>GAMSAADEVDGLGVARPHYGSVLDNERLTAEEMDERRRQNVAYEYLCHLEEAKRWMEACLGEDLPPTTELEEGLRNGVYLAKLGNFFSPKVVSLKKIYDREQTRYKATGLHFRHTDNVIQWLNAMDEIGLPKIFYPETTDIYDRKNMPRCIYCIHALSLYLFKL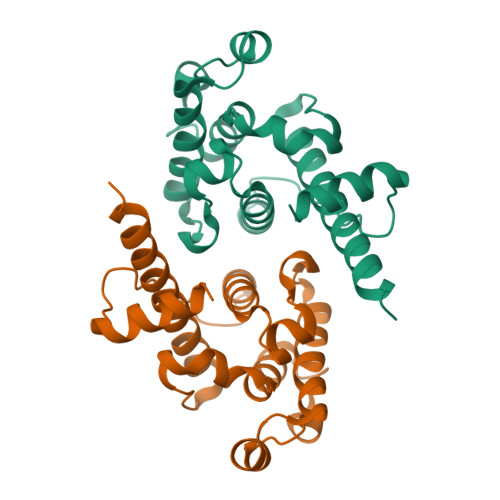GLAPQIQDLYGKVDFTEEEINNMKTELEK[4x]>SNAMKIALINENSQASKNHIIYDSLKEATDKKGYQLFNYGMRGEEGESQLTYVQNGLMAAILLNTKAVDFVVTGCGTGVGAMLALNSFPGVVCGLAVDPTDAYLYSQINGGNALSIPYAKGFGWGAELTLKLMFERLFAEEMGGGYPRERVIPEQRNARILNEVKQITHNDLMTILK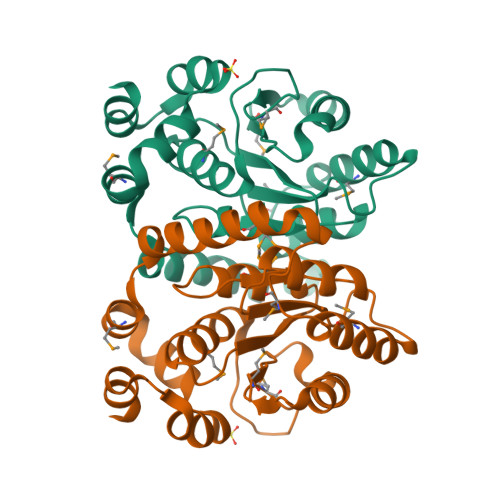IIDQDFLKDTISGKYFQEYFFENCQDDEVAAYLKEVLAK[2x]> MVFKKVLLTGTSEESFTAAADDAIDRAEDTLDNVVWAEVVDQGVEIGAVEERTYQTEVQVAFELDGS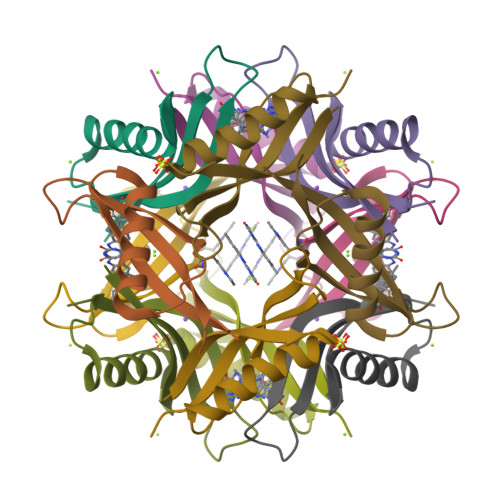QLEHHHHHH>[4x]MAQLSGQPVVILPEGTQRYVGRDAQRLNILAARIIAETVRTTLGPKGMDKMLVDSLGDIVVTNDCATILDKIDLQHPAAKMMVEVAKTQDKEAGDGTTTAVVIAGELLRKAEELLDQNIHPSIITKGYALAAEKAQEILDEIAIRVDPDDEETLLKIAATSITGKNAESHKELLAKLAVEAVKQVAEKKDGKYVVDLDNIKFEKKAGEGVEESELVRGVVIDKEVVHPRMPKRVENAKIALINEALEVKK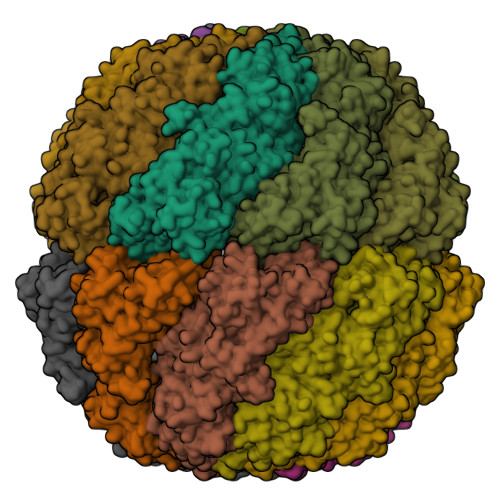TETDAKINITSPDQLMSFLEQEEKMLKDMVDHIAQTGANVVFVQKGIDDLAQHYLAKYGIMAVRRVKKSDMEKLAKATGAKIVTNVKDLTPEDLGYAEVVEERKLAGENMIFVEGCKNPKAVTILIRGGTEHVIDEVERALEDAVKVVKDVMEDGAVLPAGGAPEIELAIRLDEYAKQVGGKEALAIENFADALKIIPKTLAENAGLDTVEMLVKVISEHKNRGLGIGIDVFEGKPADMLEKGIIEPLRVKKQAIKSASEAAIMILRIDDVIAAKATKPEGGQGGGMPGGMGGMDMGM PHOSPHONIC ACIDMONO-(2-AMINO-5,6-DIMERCAPTO-4-OXO-3,7,8A,9,10,10A-HEXAHYDRO-4H-8-OXA-1,3,9,10-TETRAAZA-ANTHRACEN-7-YLMETHYL)ESTER | C10 H14 N5 O6 P S2 | 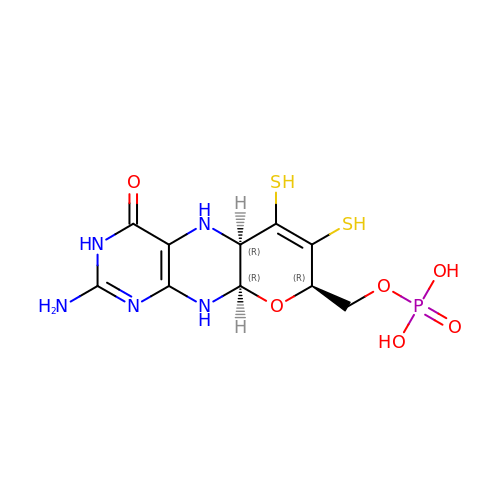HPEUEJRPDGMIMY-IFQPEPLCSA-N>[2x]GS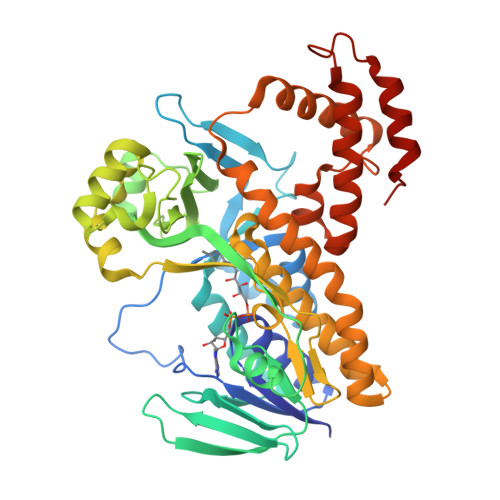MTATDNARQVTIIGAGLAGTLVARLLARNGWQVNLFERRPDPRIETGARGRSINLALAERGAHALRLAGLEREVLAEAVMMRGRMVHVPGTPPNLQPYGRDDSEVIWSINRDRLNRILLDGAEAAGASIHFNLGLDSVDFARQRLTLSNVSGERLEKRFHLLIGADGCNSAVRQAMASVVDLGEHLETQPHGYKELQITPEASAQFNLEPNALHIWPHGDYMCIALPNLDRSFTVTLFLHHQSPAAQPASPSFAQLVDGHAARRFFQRQFPDLSPMLDSLEQDFEHHPTGKLATLRLTTWHVGGQAVLLGDAAHPMVPFHGQGMNCALEDAVALAEHLQSAADNASALAAFTAQRQPDALAIQAMALENYVEMSSKVASPTYLLERELGQIMAQRQPTRFIPRYSMVTFSRLPYAQAMARGQIQEQLLKFAVANHSDLTSINLDAVEHEVTRCLPPLSHLS> PADLSGTWTLLSSDNFEGYMLALGIDFATRKIAKLLKPQKVIEQNGDSFTIHTNSSLRNYFVKFKVGEEFDEDNRGLDNRKCKSLVIWDNDRLTCIQKGE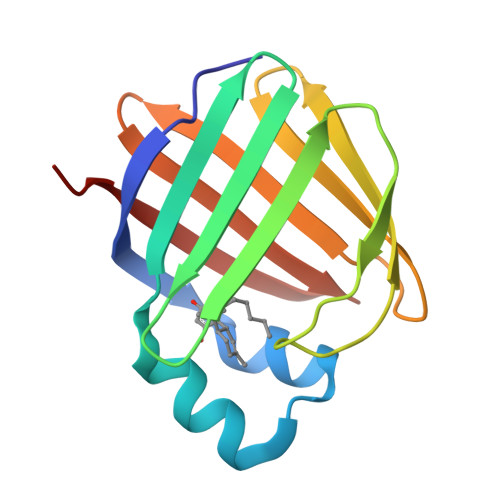KKNRGWTHWIEGDKLHLEMFCEGQVCKQTFQRALVPR>[4x]XVDSVYRTRSLGVAAEGIPDQYADGEAARVWQLYIGDTRSRTAEYKAWLLGLLRQHGCHRVLDVACGTGVDSIMLVEEGFSVTSVDASDKMLKYALKERWNRRKEPAFDKWVIEEANWLTLD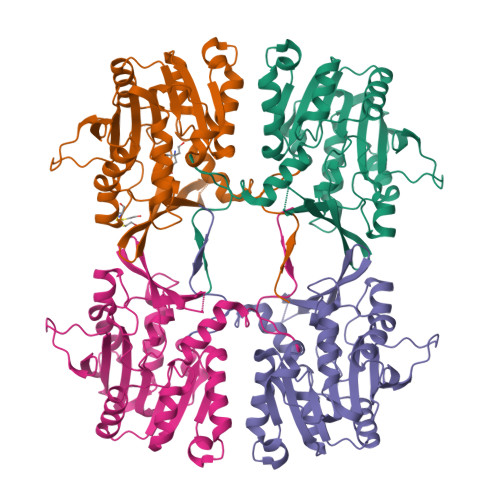KDVPAGDGFDAVICLGNSFAHLPDSKGDQSEHRLALKNIASMVRPGGLLVIDHRNYDYILSTGCAPPGKNIYYKSDLTKDITTSVLTVNNKAHMVTLDYTVQVPGAGRDGAPGFSKFRLSYYPHCLASFTELVQEAFGGRCQHSVLGDFKPYRPGQAYVPCYFIHVLKKTG;>[2x]XEEEEE> AGAGAAIAUCUUCUCU

A long-standing challenge in primordial nonenzymatic RNA copying chemistry is the biased incorporation of C and G over A and U due to differences in base pair strength. We hypothesized that 2-thiopyrimidine substitution could help overcome this bias since A:s2 U is a stronger version of the A:U base pair, and I:s2 C is a weaker version of the G:C base pair. This study explores the efficacy of a potentially primordial genetic alphabet consisting of s2 U, s2 C, A, and I. Our results show that A:s2 U and I:s2 C pairs are isoenergetic and isomorphic. All seven oligonucleotides crystallized within 2 to 3 d at 20 °C under their optimal crystallization conditions, and we solved their structures by X-ray diffraction at resolutions ranging from 1.3 to 1.6 Å.

Similarly, the sequence GCS2, 5′-AGA GAA GAU s2CUU CUC U-3′ (25), can form two G:s2C base pairs from the underlined nucleotides, near the middle of the sequence, while the sequence ICS2, 5′-AGA GAA IAU s2CUU CUC U-3′ (26), can form two I:s2C pairs at the same positions. The I:s2C base pairs in the ICS1 and ICS2 sequences exhibit only two hydrogen bonds between O6–N4 and N1–N3, due to the lack of a 2-amino group on inosine. These two hydrogen bonds are located at the same position and have similar bond lengths as in the A:s2U base pair. The superimposed I:s2C and A:s2U pairs show that these two base pairs are isomorphic. The missing hydrogen bond is presumably the main reason that the I:s2C pair is weaker than the Watson–Crick G:C pair. However, the hydrogen bond between N1 on I and N3 on s2C has a slightly shorter length (2.7 Å) than both Watson–Crick G:C pair (2.9 Å) and G:s2C pair (3.0 Å). This stronger hydrogen bond may partially compensate for the loss of enthalpy due to the missing third hydrogen bond. In contrast, the absence of the 2-amino group on inosine and lack of an N2–S2 hydrogen bond results in the I:s2C base pair exhibiting no significant changes in the base pair opening angle, thereby making it possible to enhance the N1–N3 hydrogen bond. The distances between C2 on I or A and S2 on s2C or s2U in all structures containing I:s2C or A:s2U base pairs are consistently 3.5 to 3.6 Å, falling within the typical range for a C–H⋯S hydrogen bond. This suggests that a third hydrogen bond may form in both the I:s2C and A:s2U base pairs, but not in the I:C or A:U pairs.>[7x]AEPVYPDQLRLFSLGQGVCGDKYRPVNREEAQSVKSNIVGMMGQWQISGLANGWVIMGPGYNGEIKPGTASNTWCYPTNPVTGEIPTLSALDIPDGDEVDVQWRLVHDSANFIKPTSYLAHYLGYAWVGGNHSQYVGEDMDVTRDGDGWVIRGNNDGGCDGYRCGDKTAIKVSNFAYNLDPDSFKHGDVTQSDRQLVKTVVGWAVNDSDTPQSGYDVTLRYDTATNWSKTNTYGLSEKVTTKNKFKWPLVGETELSIEIAANQSWASQNGGSTTTSLSQSVRPTVPARSKIPVKIELYKADISYPYEFKADVSYDLTLSGFLRWGGNAWYTHPDNRPNWNHTFVIGPYKDKASSIRYQWDKRYIPGEVKWWDWNWTIQQNGLSTMQNNLARVLRPVRAGITGDFSAESQFAGNIEIGAPVPLAA

Aerolysin is a major contributor to the pathogenicity of Aeromonas spp, which causes gastroenteritis, deep wound infections and sepsis in humans. It is a pore-forming toxin (PFT), which is secreted by the bacterium as a water-soluble protein, binds receptors on their target cell membrane and, following proteolytic activation, forms circular heptameric oligomers that insert into the plasma membrane thus permeabilizing it, potentially leading to cell death. Aerolysin belongs to the family of β-PFTs, meaning that the final pore spans the membrane in the form of a β-barrel and defines the aerolysin-like family of proteins that share a common structural motif3. Combined, these structures, consistent with the recent lysenin pore structure, describe the major steps involved in the pore-formation process by aerolysin: the transition from the monomer to the oligomer with the formation of two highly stable concentric β-barrels, the zipper-like formation of the β-barrel and the final piston-like puncturing of the lipid bilayer.

To verify that the quasipore conformation is indeed representative of the full pore conformation, we analysed the structure of wild-type aerolysin heptamers. If performed at sufficiently low aerolysin concentration, it allowed us to reduce aggregation and to obtain relatively well-dispersed individual pores in detergent micelles. Cryo-EM analysis led to a 7.9 Å resolution map of the wild-type pore. This resolution was sufficient to fit the quasipore model by rigid-body docking, demonstrating that it very closely corresponds the wild-type final pore density map. Most interestingly, the nine amino acids at the tip of each β-hairpins adopt a different conformation than in anthrax protective antigen and fold sideways in a rivet-like fashion, confirming our previous experimental conclusions. Similarly, to other transmembrane β-barrels, including the lysenin pore13, the position of two rings of aromatic residues spaced by 32 Å delineate the edge of the transmembrane regions (highlighted in Fig. 4a). The extended inner β-barrel of the pore is 87 Å long, spanning the entire length of the protein. Once in the membrane, each loop formed by nine amino acids at the tip of the inner β-barrel folds sideways and lies approximately parallel to the membrane plane, leading to a rivet-like anchoring.>ASRGVNKVILVGNLGQDPEVRYMPNGGAVANITLATSESWRDKATGEMKEQTEWHRVVLFGKLAEVASEYLRKGSQVYIEGQLRTRKWTDQSGQDRYTTEVVVNVGGTMQMLGGRQGGGAPAGGNIGGGQPQGG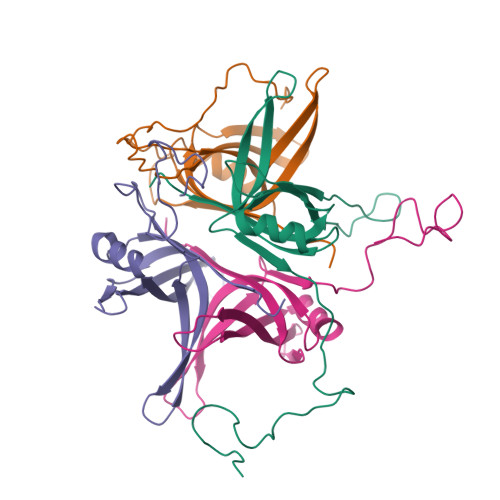WGQPQQPQGGN[4x]3,6-BIS(METHYLENE)DECANOIC ACID | C12 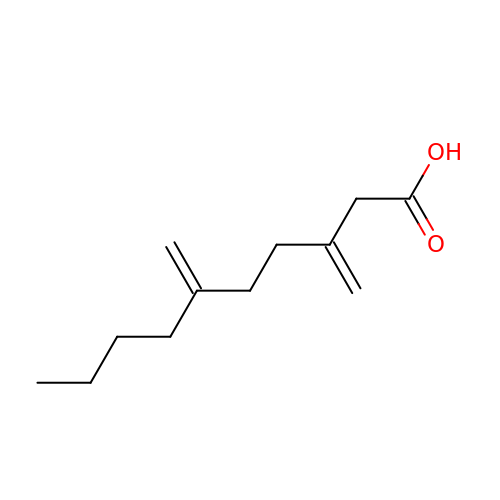H20 O2 | YOHXQMVSYCADHX-UHFFFAOYSA-N>MDQETIDTDYDVIVLGTGITECILSGLLSVDGKKVLHIDKQDHYGGEAASVTLSQLYEKFKQNPISKEERESKFGKDRDWNVDLIPKFLMANGELTNILIHTDVTRYVDFKQVSGSYVFKQGKIYKVPANEIEAISSPLMGIFEKRRMKKFLEWISSYKEDDLSTHQGLDLDKNTMDEVYYKFGLGNSTKEFIGHAMALWTNDDYLQQPARPSFERILLYCQSVARYGKSPYLYPMYGLGELPQGFARLSAIYGGTYMLDTPIDEVLYKKDTGKFEGVKTKLGTFKAPLVIADPTYFPEKCKSTGQRVIRAICILNHPVPNTSNADSLQIIIPQSQLGRKSDIYVAIVSDAHNVCSKGHYLAIISTIIETDKPHIELEPAFKLLGPIEEKFMGIAELFEPREDGSKDNIYLSRS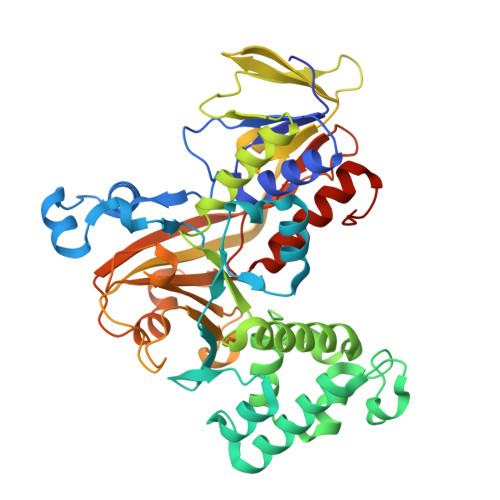YDASSHFESMTDDVKDIYFRVTGHPLVLKQRQEQEKQ[2x]>[2x]MKLLQRGVALALLTTFTLASETALAYEQDKTYKITVLHTNDHHGHFWRNEYGEYGLAAQKTLVDGIRKEVAAEGGSVLLLSGGDINTGVPESDLQDAEPDFRGMNLVGYDAMAIGNHEFDNPLTVLRQQEKWAKFPLLSANIYQKSTGERLFKPWALFKRQDLKIAVIGLTTDDTAKIGNPEYFTDIEFRKPADEAKLVIQELQQTEKPDIIIAATHMGHYDNGEHGSNAPGDVEMARALPAGSLAMIVGGHSQDPVCMAAENKKQVDYVPGTPCKPDQQNGIWIVQAHEWGKYVGRADFEFRNGEMKMVNYQLIPVNLKKKVTWEDGKSERVLYTPEIAENQQMISLLSPFQNKGKAQLEVKIGETNGRLEGDRDKVRFVQTNMGRLILAAQMDRTGADFAVMSGGGIRDSIEAGDISYKNVLKVQPFGNVVVYADMTGKEVIDYLTAVAQMKPDSGAYPQFANVSFVAKDGKLNDL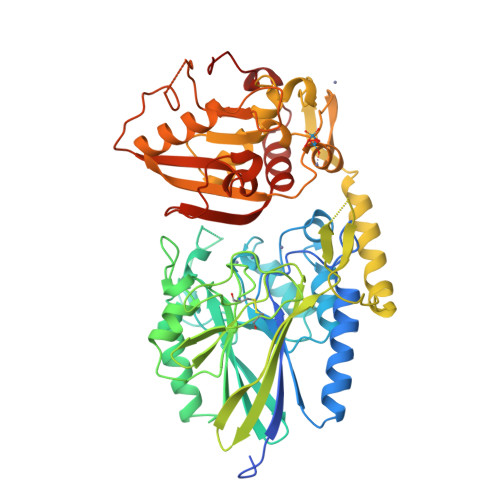KIKGEPVDPAKTYRMATLNFNATGGDGYPRLDNKPGYVNTGFIDAEVLKAYIQKSSPLDVSVYEPKGEVSWQ>[2x]MGSERTCCPVNWVEHERSCYWFSRSGKAWADADNYCRLEDAHLVVVTSWEEQKFVQHHIGPVNTWMGLHDQNGPWKWVDGTDYETGFKN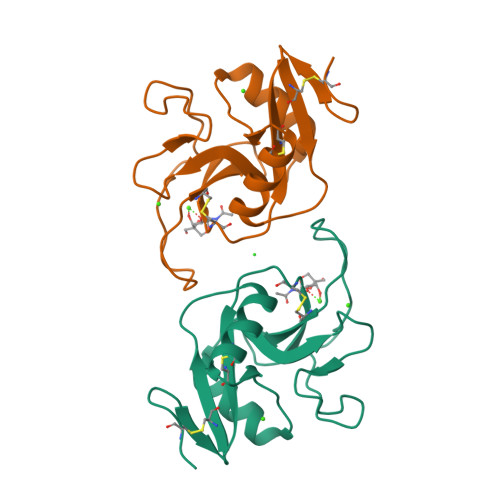WRPEQPDDWYGHGLGGGEDCAHFTDDGRWNDDVCQRPYRWVCETELDKASQEPPLL> QLTPTFYDNSCPNVSNIVRDTIVNELRSDPRIAASILRLHFHDCFVNGCDASILLDNTTSFRTEKDAFGNANSARGFPVIDRMKAA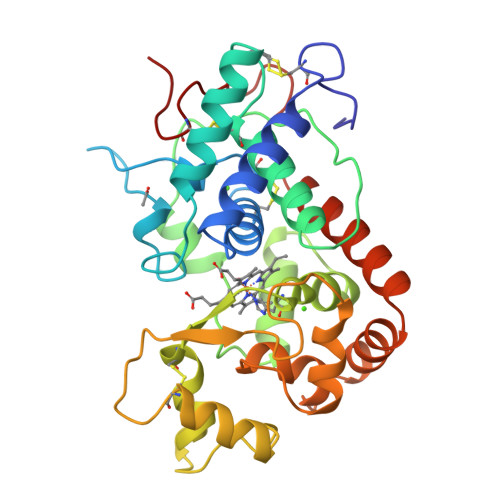VESACPRTVSCADLLTIAAQQSVTLAGGPSWRVPLGRRDSLQAFLDLANANLPAPFFTLPQLKDSFRNVGLNRSSDLVALSGGHTFGKNQCRFIMDRLYNFSNTGLPDPTLNTTYLQTLRGLCPLNGNLSALVDFDLRTPTIFDNKYYVNLEEQKGLIQSDQELFSSPNATDTIPLVRSFANSTQTFFNAFVEAMDRMGNITPLTGTQGQIRLNCRVVNS> KKHSVLHLVPVNITSKADSDVTEVMWQPVLRRGRGLEAQGDIVRVWDTGIYLL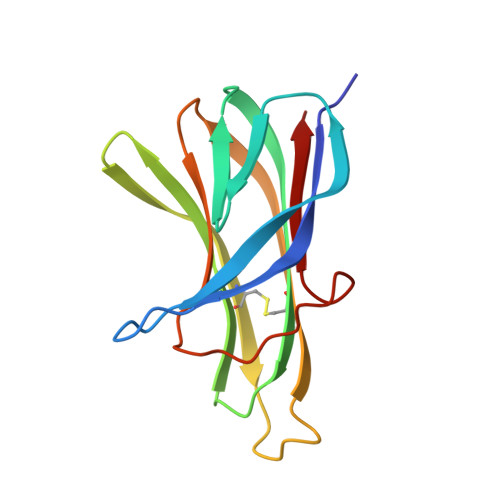YSQVLFHDVTFTMGQVVSREGQGRRETLFRCIRSMPSDPDRAYNSCYSAGVFHLHQGDIITVKIPRANAKLSLSPHGTFLGFVKL>[4x]MYLTKEEELILAGEYGYALQKAMEILVALGDIYGADRLIPIKSAQVAGVSYKNIGDAGIEFLRDFVEAGAKVSVYTTLNPAGIGDDEFMEKQMEVLELYRKMGIEVTSTCTPYYGANLPKFGDHIAWSESSAVSFANSILGARTNREGGPSSLAAAIVGKTPNYGLHLDENRKATVIVDVKAKVKTFADYSVLGYHVGKTLGNDVPYFKNLKPEKTEFLKELGAAMGATGSIALYHVEGETPEYREAITDKLETITVEDSDLKAVRESFQDDWSDIDMILIGCPHASLPEVKEIAELLRMRGKPLKIPLFITASRAVKALADALGYTEIIERYNGKIIPDSCFVVSPIKGWYRGIATNSGKSAFYFRSFGFSVRLDDVENLIKEAP;>[4x]GPKLKGRKIVGGKAEGEVIVSRKPLSFLGGVDPETGIVTDAESDIRGQSIAGKILVFPRGKGSTVGSYVIYALKKNNKAPKAIIVGEAETIVATGAIISDIPMVDGVDVSKLKTGMKVRVDADSGEVEILEDGE

Aconitase superfamily members catalyze the homologous isomerization of specific substrates by sequential dehydration and hydration and contain a [4Fe-4S] cluster. However, monomeric and heterodimeric types of function unknown aconitase X (AcnX) have recently been characterized as a cis-3-hydroxy-L-proline dehydratase (AcnXType-I) and mevalonate 5-phosphate dehydratase (AcnXType-II), respectively. We herein elucidated the crystal structures of AcnXType-I from Agrobacterium tumefaciens (AtAcnX) and AcnXType-II from Thermococcus kodakarensis (TkAcnX) without a ligand and in complex with substrates. AtAcnX and TkAcnX contained the [2Fe-2S] and [3Fe-4S] clusters, respectively, conforming to UV and EPR spectroscopy analyses.

Therefore, to elucidate the catalytic mechanism at the atomic level, we performed a crystallographic analysis of AcnXType-IIb from TkAcnX; the small and large subunits (TkAcnXS and TkAcnXL) showed sequence identities of 43% and 37% with those of ApAcnX, respectively. The crystal structure of TkAcnX in the apo-form was elucidated at 3.4 Å by molecular replacement using the coordinate set for the structure of AtAcnX in the apo-form; recombinant ApAcnX was also originally prepared, but not crystallized. The crystallographic asymmetric unit contained four TkAcnX molecules consisting of four chains of TkAcnXS (chains B, D, F, and H) and four chains of TkAcnXL (chains A, C, E, and G), the conformations of which (except for the chain B) were very similar; r.m.s.d. values on the Cα atoms were 0.36–0.42 and 0.29–0.37 Å, respectively. As expected from the primary structure, each TkAcnXS (residues 1–130) and TkAcnXL subunit (residues 1–386) superimposed well on residues 1–144 and 157–558 of AtAcnX, with r.m.s.d. values of 1.3 Å over 122 Cα atoms and 1.6 Å over 372 Cα atoms, respectively. Small differences in folding were only observed in TkAcnXS; the N-terminal region formed an additional β-strand (β1), by which the β-barrel was created by nine β-strands, and a shorter loop was connected between β9 and β10 instead of α3 in AtAcnX. On the other hand, the heterodimeric structure of TkAcnX showed a more “opened” conformation than that of AtAcnX. The electron density map and anomalous difference Fourier map suggested that TkAcnX has a cuboidal [3Fe-4S] cluster. Fe1, Fe3, and Fe4 atoms were ligated to the protein by Cys110(L), Cys342(L), and Cys283(L), respectively (the letters in parentheses indicate the location in the subunit). On the other hand, among the [Fe-S] cluster-binding sites, only Cys110(L) (yellow-green) and Cys342(L) (green) were homologous to Cys273 and Cys508 in AtAcnX, respectively, whereas Cys283(L) (aqua) corresponded to Cys358 in mAcn. Although the crystal structure(s) of TkAcnX elucidated in the present study corresponded to the inactive form, in hypothetically activated TkAcnX, the Fe2 atom in the [4Fe-4S] cluster may interact with a water molecule, Glu129(L), and Lys361(L) as well as AtAcnX.> MTNIEPVIIETRLELIGRYLDHLKKFENISLDDYLSSFEQQLIT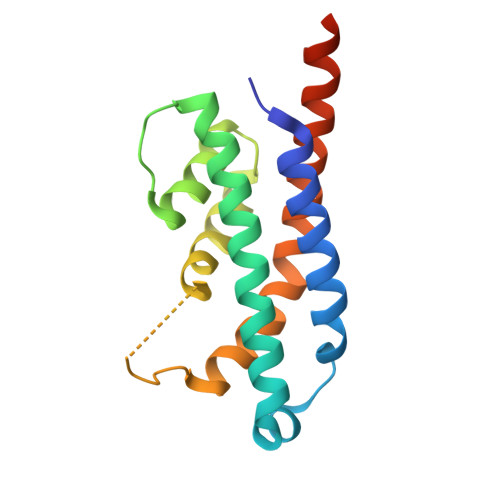EELLQLITQAAIDINDHILSKLKSGKSYTNFEAFIELGKYQILTPELAKQIAPSSGLRNRLVHEYDDIDPNQVFMAISFALQQYPLYVRQINSYLITLEEENDLESGHHHHHH>[2x]MDSKYQCVKLNDGHFMPVLGFGTYAPAEVPKSKALEATKLAIEAGFRHIDSAHLYNNEEQVGLAIRSKIADGSVKREDIFYTSKLW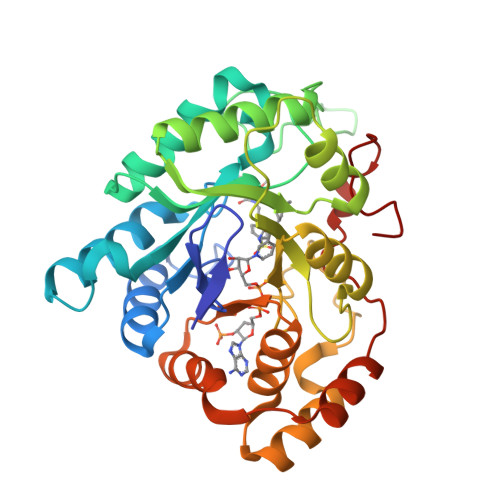CNSHRPELVRPALERSLKNLQLDYVDLYLIHFPVSVKPGEEVIPKDENGKILFDTVDLCATWEAVEKCKDAGLAKSIGVSNFNRRQLEMILNKPGLKYKPVCNQVECHPYFNQRKLLDFCKSKDIVLVAYSALGSHREEPWVDPNSPVLLEDPVLCALAKKHKRTPALIALRYQLQRGVVVLAKSYNEQRIRQNVQVFEFQLTSEEMKAIDGLNRNVRYLTLDIFAGPPNYPFSDEY> HXEGCF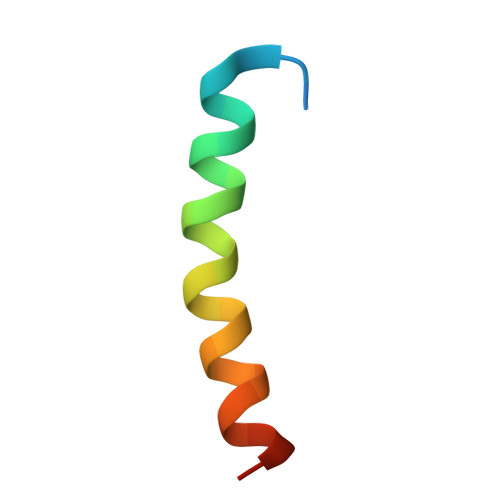TSDVSSYLEGQAAKEFIAWLVKGRG> MDPSLVLEQTIQDVSNLPSEFRYLLEEIGSNDLKLIEEKKKYEQKESQIHKFIRQQGSIPKHPQEDGLDKEIKESLLKCQSLQREK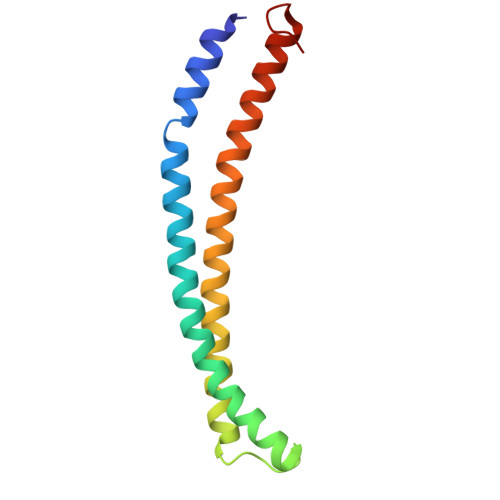CVLANTALFLIARHLNKLEKNIALLEEDGVLAPV Second, the ribonucleoprotein telomerase elongates shortened telomeres at chromosomal ends using a reverse transcriptase activity. Although the human telomerase holoenzyme is composed of multiple accessory subunits, catalysis is localized to the telomerase reverse transcriptase (TERT) subunit. We found that, in terms of global protein structure, minimal rearrangement is required to proceed through the catalytic cycle.

We determined how TERT engages with telomeric DNA by co-crystallizing tcTERT with a 16-mer RNA strand hybridized to its complementary 15-mer DNA strand to form a binary complex. This substrate mimics the initial TERT:RNA complex bound to telomeric DNA (state A6). In this orientation, an unpaired 5’ cytosine (rC) of the RNA strand acts as the templating base and a 3’ adenosine (dA) of the DNA strand serves as the primer terminus. Crystals of this complex grew in a P3221 space group, diffracting to 2.5 Å resolution. The resulting structure shows TERT bound as a ring around the end of the RNA:DNA complex, with its active site positioned at the terminus of the DNA strand. Residues I196, V197, S198, G309, and R194 compose a pocket around the templating RNA base. This pocket uses both polar and nonpolar interactions to stabilize the templating rC in a conformation that orients its Watson-Crick edge towards the incoming nucleotide binding site. On the opposite side, the 3’-OH of the primer terminal 3’-dA points towards the catalytic metal binding site, and side chains from T341 and V342 coordinate the deoxyribose sugar moiety of the 3’-dA with nonpolar interactions. This binary TERT complex also has a cavity in the active site that forms the nucleotide binding pocket. Collectively, the active site of tcTERT is primed for nucleotide binding, and the residues involved in binding are highly conserved with human telomerase.

> GMVHYYRLSLKSRQKAPKIVNSKYNSILNIALKNFRLCKKHKTKKPVQILALLQEIIPKSYFGTTTNLKRFYKVVEKILTQSSFECIHLSVLHKCYDYDAIPWLQNVEPNLRPKLLLKHNLFLLDNIVKPIIAFYYKPIKTLNGHEIKFIRKEEYISFESKVFHKLKKMKYLVEVQDEVKPRGVLNIIPKQDNFRAIVSIFPDSARKPFFKLLTSKIYKVLEEKYKTSGSLYTCWSEFTQKTQGQIYGIKVDIRDAYGNVKIPVLCKLIQSIPTHLLDSEKKNFIVDHISNQFVAFRRKIYKWNHGLLQGDPLSGCLCELYMAFMDRLYFSNLDKDAFIHRTVDDYFFCSPHPHKVYDFELLIKGVYQVNPTKTRTNLPTHRHPQDEIPYCGKIFNLTTRQVRTLYKLPPNYEIRHKFKLWNFNNQISDDNPARFLQKAMDFPFICNSFTKFEFNTVFNDQRTVFANFYDAMICVAYKFDAAMMALRTSFLVNDFGFIWLVLSSTVRAYASRAFKKIVTYKGGKYRKVTFQCLKSIAWRAFLAVLKRRTEIYKGLIDRIKSREKLTMKFHDGEVDASYFCKLPEKFRFVKINRKASI2,3-DICARBOXY-4-(2-CHLORO-PHENYL)-1-ETHYL-5-ISOPROPOXYCARBONYL-6-METHYL-PYRIDINIUM 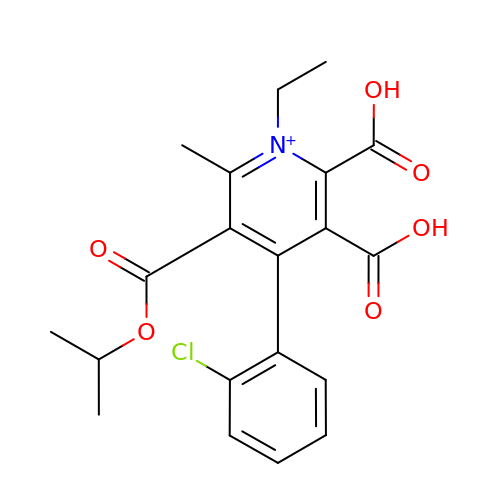| C20 H21 Cl N O6 | HMSIYRVIPQHZBI-UHFFFAOYSA-O>[2x]GSMERKRWECPALPQGWEREEV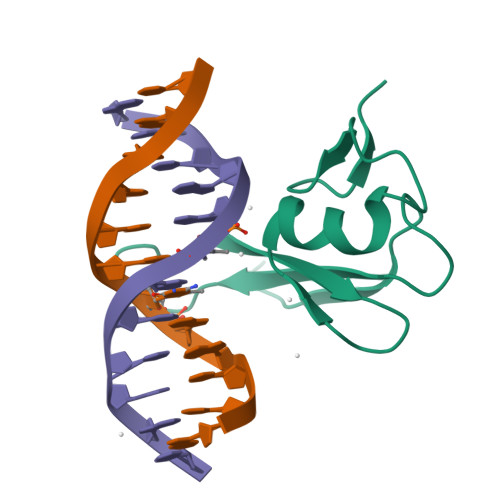PRRSGLSAGHRDVFYYSPSGKKFRSKPQLARYLGGSMDLSTFDFRTGKMLM> MDEEYDVIVLGTGLTECILSGIMSVNGKKVLHMDRNPYYGGESSSITPLEELYKRFQLLEGPPETMGRGRDWNVDLIPKFLMANGQLVKMLLYTEVTRYLDFKVVEGSFVYKGGKIYKVPSTETEALASNLMGMFEKRRFRKFLVFVANFDENDPKTFEGVDPQNTSMRDVYRKFDLGQDVIDFTGHALALYRTDDYLDQPCLETINRIKLYSESLARYGKSPYLYPLYGLGELPQGFARLSAIYGGTYMLNKPVDDIIMENGKVVGVKSEGEVARCKQLICDPSYVPDRVRKAGQVIRIICILSHPIKNTNDANSCQIIIPQNQVNRKSDIYVCMISYAHNVAAQGKYIAIASTTVETTDPEKEVEPALELLEPIDQKFVAISDLYEPIDDGSESQVFCSCSYDATTHFETTCNDIKDIYKRMAGSAFDF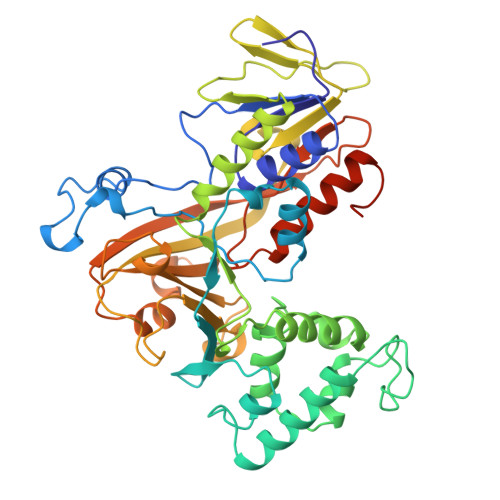ENMKRKQNDVFGEADQ> GMS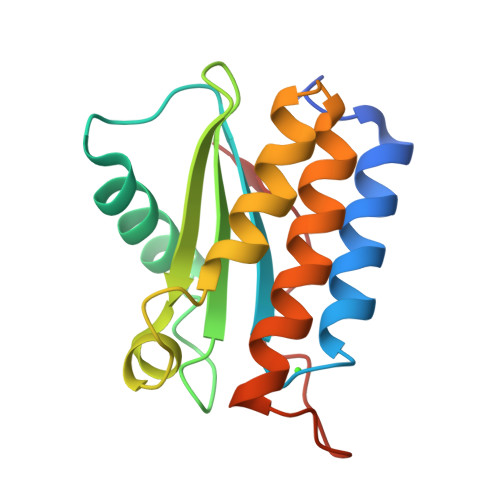KIEEFLTAEEEKAIVDAIRDAEKNTSGEIRVHLEKTSEIDVFDRAMDVFHNLKMDNTKLQNGVLIYVAVEDKTFVIYGDKGINDVVSDDFWDTTRNAIQLQFKQGNFKQGLVDGIEKAGMALAKYFPWKKDDIDELPNTISKG>[2x]VHINKGGRPRQHLLSLTRRAQKHRLRELKIQVKEFADKEEGGDVKAVCLTLFLLALRARNEHRQADELEAIMQGRGSGLQPAVCLAIRVNTFLSCSQYHKMYRTVKAITGRQIFQPLHALRNAEKVLLPGYHPFEWQPPLKNVSSRTDVGIIDGLSGLASSVDEYPVDTIAKRFRYDSALVSALMDMEEDILEGMRSQDLDDYLNGPFTVVVKESCDGMGDVSEKHGSGPAVPEKAVRFSFTVMRITIEHGSQNVKVFEEPKPNSELCCKPLCLMLADESDHETLTAILSPLIAEREAMKSSELTLEMGGIPRTFKFIFRGTGYDEKLVREVEGLEASGSVYICTLCDTTRLEASQNLVFHSITRSHAENLQRYEVWRSNPYHESVEELRDRVKGVSAKPFIETVPSIDALHCDIGNAAEFYKIFQLEIGEVYKHPNASKEERKRWQATLDKHLRKRMNLKPIMRMNGNFARKLMTQETVDAVCELIPSEERHEALRELMDLYLKMKPVWRSSCPAKECPESLCQYSFNSQRFAELLSTKFKYRYEGKITNYFHKTLAHVPEIIERDGSIGAWASEGNQSGNKLFRRFRKMNARQSKCYEMEDVLKHHWLYTSKYLQKFMNAHNA;>[2x]MSLQMVTVGHNIALIQPGFSLMNFDGQVF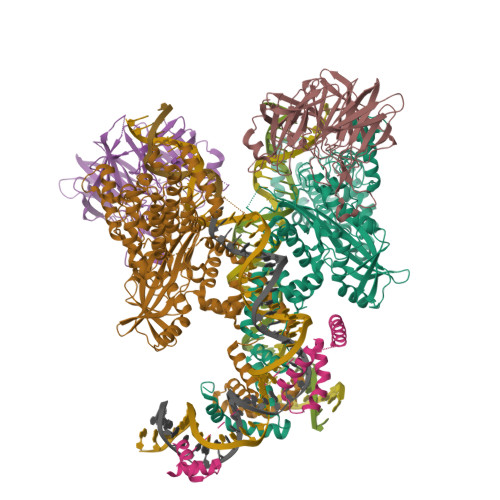FFGQKGWPKRSCPTGVFHFDIKQNHLKLKPAIFSKDSCYLPPLRYPATCSYKGSIDSDKHQYIIHGGKTPNNELSDKIYIMSVACKNNKKVTFRCTEKDLVGDVPEPRYGHSIDVVYSRGKSMGVLFGGRSYMPSTQRTTEKWNSVADCLPHVFLIDFEFGCATSYILPELQDGLSFHVSIARNDTVYILGGHSLASNIRPANLYRIRVDLPLGTPAVNCTVLPGGISVSSAILTQTNNDEFVIVGGYQLENQKRMVCSLVSLGDNTIEISEMETPDWTSDIKHSKIWFGSNMGNGTIFLGIPGDNKQAMSEAFYFYTLRCSEEDLSEDQ;> MGKGDPKKPRGKMSSYAFFVQTCREEHKKKHPDASVNFSEFSKKCSERWKTMSAKEKGKFEDMAKADKARYEREMKTYIPPKGETKKKFKDPNAPKRPPSAFFLFCSEYRPKIKGEHPGLSIGDVAKKLGEMWNNTAADDKQPYEKKAAKLKEKYEKDIAAYR>[2x]SMAKAKAPRRTLDSYTVKPINKTVKPGDCVLMRPSDPSKPSYVAKIERIESDGRGPNVRVRVRWYYRPEESIGGRRQFHGSKEVFLSDHYDTQSADTIEGKCMVHSFKNYTKLDAVGNDDFFCRFEYNSSTGAFNPDRVAVYCKCEMPYNPDDLMVQCEGCSDWFHPACIEMSAEEAKRLDHFFCENCSSEGQKKLQNSHNTRQSDAKAETKRRRR;>LATKAARKSAPATGGVK[2x]

In Arabidopsis, the BAH and PHD dual domain-containing proteins SHORT LIFE (SHL) and EARLY BOLTING IN SHORT DAYS (EBS) function in chromatin-mediated floral repression and seed dormancy. Here, our biochemical and X-ray structural studies show that SHL is capable of recognizing an active histone mark H3K4me3 and a repressive mark H3K27me3 independently via its PHD and BAH domain, respectively. In this study, we identified SHL as a dual histone methyl-lysine reader that is distinct from other reader proteins in recognizing both H3K4me3 and H3K27me3, two well-known histone marks with opposing roles in balancing chromatin and transcriptional states. In contrast, the SHL from Populus trichocarpa (PtSHL), which has similar PHD and BAH domains and shows similar H3K4me3 and H3K27me3-binding affinities, successfully yielded crystals.

We further determined the structure of the PtSHL-H3(20–36)K27me3 complex at 3.2 Å resolution. The peptide adopts a right angle-like conformation with a sharp turn at H3A31 and is bound within a negatively charged surface cleft on the BAH domain. In detail, the interaction features the recognition of the H3K27me3 trimethyllysine by a classical aromatic cage formed by Tyr41, Trp63, and Tyr65, similar to other canonical methyl-lysine readers. Interestingly, the side chain hydroxyl group of H3S28 is anchored and fixed between PtSHL His88 and Asp90 and forms two hydrogen bonds with them. The interaction between H3S28 and PtSHL His88 fixes the side chain rotamer of His88, locking the conformation of the imidazole ring of His88 in a parallel alignment with the prolyl ring of H3P30 with the alignment stabilized by hydrophobic and CH–π interactions. Although H3K9 and H3K27 share the ARKS consensus motif, H3P30 at the n + 3 position of H3K27me3 (but not H3G12 at the n + 3 position of H3K9me3) can be specifically recognized by PtSHL, suggesting a sequence-specific recognition mechanism. Mutations of His88 (H88A) or Asp90 (D90A) involved in H3P30 recognition as well as mutations of the aromatic residues responsible for H3K27me3 recognition (Y41A, W63A, Y65A), abolished the binding of PtSHL with H3K27me3. In addition, Arg32, Asp90, Gln92, and Asp95 form several hydrogen bonds with the main chain of the bound H3K27me3 peptide. The superposition of the two complexes yields an RMSD of 0.94 Å, suggesting a nearly identical overall structures. Moreover, the binding between 2-fold excess H3(1–15)K4me3 pre-saturated PtSHL and H3(20–36)K27me3 yielded a binding affinity of 18.7 μM, similar to the 21.3 μM binding between PtSHL and H3K27me3, suggesting that the recognition of H3K4me3 by the PHD finger and the recognition of H3K27me3 by the BAH domain are independent of each other.In this study, we identified four enzymes (two GH183 endo-d-arabinanases, GH172 exo-α-d-arabinofuranosidase, and GH116 exo-β-d-arabinofuranosidase) from Microbacterium arabinogalactanolyticum. These enzymes completely degraded the complex d-arabinan core structure of lipoarabinomannan and arabinogalactan in a concerted manner. Furthermore, through biochemical characterization using synthetic substrates and X-ray crystallography, we elucidated the mechanisms of substrate recognition and anomer-retaining hydrolysis for the α- and β-d-arabinofuranosidic bonds in both endo- and exo-mode reactions. We propose a d-arabinan-degrading pathway for Mi. arabinogalactanolyticum based on its gene cluster and four characterized enzymes.

The crystal structures of ExoMA2 were determined at 1.75 and 1.35 Å resolutions for the complex forms with Tris (buffer molecule) and β-d-Araf, respectively. The two structures are almost identical (Cα RMSD < 0.19 Å for all chain pairs), and we will mainly describe the complex structure with β-d-Araf. A dimer is present in the asymmetric unit of the ExoMA2 crystal, consistent with the SEC measurement in solution and the PISA server prediction. ExoMA2 has a two-domain structure consisting of N-terminal β-sandwich and C-terminal (α/α)6 barrel domains, the latter being the catalytic domain. The two-domain structure resembles that of GH116 β-glucosidase from Thermoanaerobacterium xylanolyticum (TxGH116, Dali Z score = 42.4 and Cα RMSD = 2.5 Å), whereas the amino acid sequence identity is very low (21%). Compared with TxGH116, ExoMA2 has an additional long loop and a small β-sandwich domain in the N-terminal and C-terminal domains, respectively. In contrast, GH172 αFFase1 (anomer-retaining α-d-Araf-ase)17 initially produced α-d-Araf. This finding indicated that ExoMA2 is an anomer-retaining GH.

>[2x]MSKIKSRRARRIPHTAESVAFPLGGIGTGNVSLGARGELRDWEFENLPDKGRLNPRSFFAIHAAPQGGPSATRVLEARSSGRHDRDAGYGFDELAGLPRLDSAGLHGEYPVVDIDFTDATLPVTVSLHAFTPLVPLDADASGIPAAVLRYRVVNPGDAPVTVTVVGSMSHTAGRGAPGPDAPWGMRGTQSVRWRESDGIRGLDFDIDLDHDDPGYGTMSLTTTDSSTTVKPQWVTSYWPDGARLFWNDLADDGLLAPEARLTLEDKPRGLFAERDADPDAPALTEEQMLAKLPRVRTGSLGIVHTLAPGEERDFEFVLAWSFPNRRRGWHGHIIFDDALEDGAPDLRDELGPIVRNHYAVRWPDAWAAAAQLHRDLPALEGATDAFVEELYGGSLDPVLADAVGANIAALRSTTCFVLESPTPELGDGPVFAAWEGSFDHGGSCEGTCTHVWSYAQTAAWLFPGLERSARRAEYLLETDESGAQKFRGNRIFGAPRWFIGPAVDGQLGTFLRLHREWRFCGDDEFLRELWPAAARTLDYAAREWDHDGDGLLDGEMHNTYDIEFHGVEPLSNIIHLAALRAGVRMAGHLGDTARAQEWALRADHVAAAIEGVLWNGEYYRQVIDDVDAHRYQYGDGVLSDQLLGQFHAFLGGLGYLLPEAHVRSALDAIVQHNHRGDLRDHESTQRVYALNDEGGLLLASWPEGGRPALPFVYADEVWTGIEHQVAVSLLFAGRYDDALRIERTLRARYDGAHRSPWNEIECGNHYARSLASWGLLIGASGAQWDAGARTLSFDPVLPGDARFLFTTATGWGGVEIGDDVITLRLHGGALDLDELRLRGEVAGRGIHLDAGETRTLTLTLEHHHHHH> SNA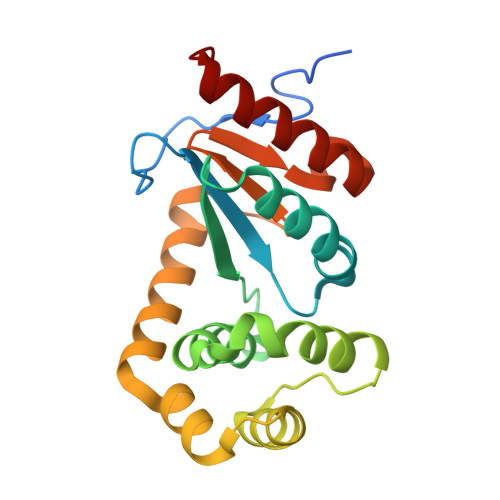AGFAQASPSAPVAGKDFEVMKSPQPVSAPAGKVEVIEFFWYGCPHAYEFEPTIEAWVKKQGDKIAFKRVPVAFRDDFVPHSKLFYALAALGVSEKVTPAVFNAIHKEKNYLLTPQAQADFLATQGVDKKKFLDAYNSFSVQGQVKQSAELLKNYNIDGVPTIVVQGKYKTGPAYTNSLEGTAQVLDFLVKQVQDKKL>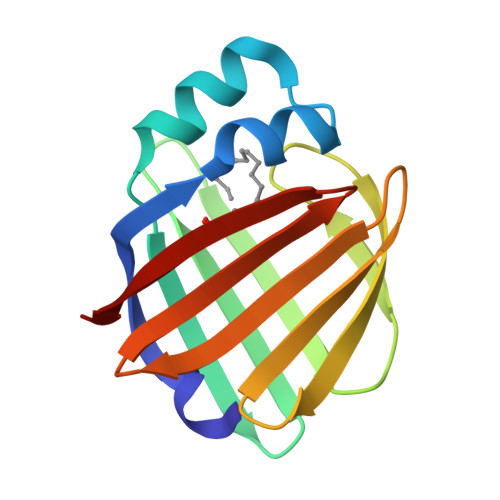AADLAGKWILESSENFDDYMKAVGVGMVMRKMANAATPTQEIKIDGDSWSIKTSTTFKTTDISFTIGQEFDETTGDGRKIKTTCKIDGNAMIQDQKGSPDSILSREVKDGKMHMILKVNDVVCTRIFKRVD[3x]> SNAMRMIDIIEKKRDGHTLTTEEINFFIGGYVKGDIPDYQASSLAMAIYFQDMNDDERVALTMAMVNSGDMIDLSDIKGVKVDKHSTGGVGDTTTLVLAPLVAAVDVPVAKMSGRGLGHTGGTIDKLEAIDGFHVEIDEATFVKLVNENKVAVVGQSGNLTPADKKLYALRDVTGTVNSIPLIASSIMSKKIAAGADAIVLDVKTGSGAFMKTLEDAEALAHAMVRIGNNVGRNTMAIISDMNQPLGRAIGNALELQEAIDTLKGQGPKDLTELVLTL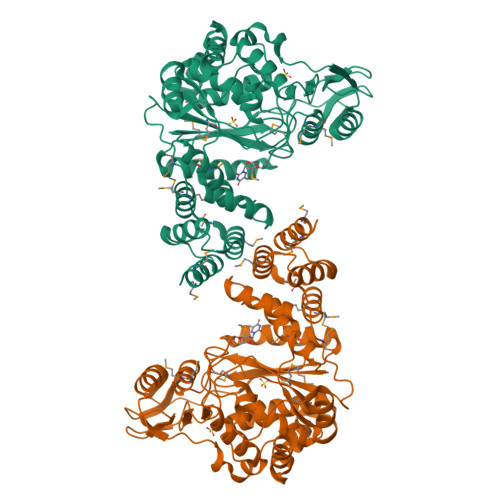GSQMVVLANKAETLEEARALLIEAINSGAALEKFKTFIKNQGGDETVIDHPERLPQAQYQIEYKAKKSGYVTELVSNDIGVASMMLGAGRLTKEDDIDLAVGIVLNKKIGDKVEEGESLLTIHSNRQDVDDVVKKLDSSITIADHVVSPTLIHKIITE7-[4-(2-aminoethyl)phenyl]-4-methylquinolin-2-amine | C18 H19 N3 | 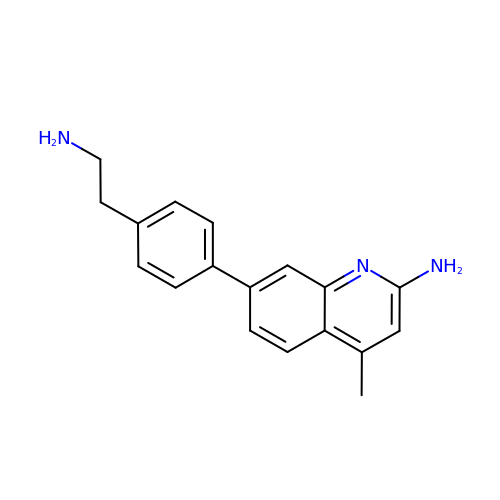JQIPWXPQEFGIOD-UHFFFAOYSA-N>GSHFEEGERVLAKHSDCFYEAKVLKVEFKDNEWKYFVHYIGWNKSWDEWIRLDCLLKHSDENIEKQKEQGLK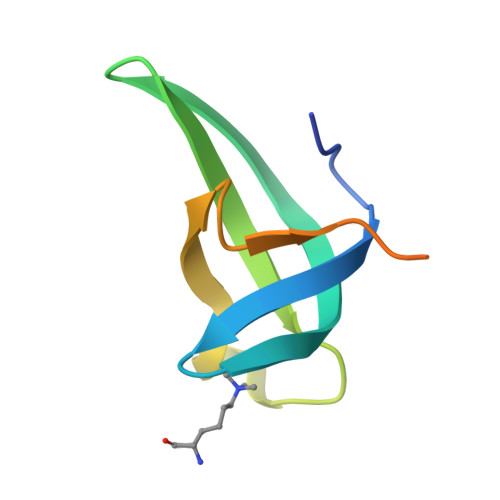QQG[2x];>[2x]ATGGVKKPHRY>[2x]GPGSTVNEQVQAWESRRPLIQDLARRLLTDDEVLAVTRHCSRYVHEGGVEDLVRPLLAILDRPTKLLLLRDIRSVVAPTDLGRFDSMVMPVELEAFEALKSRAVG

PDZ domain-containing 7 (PDZD7) is part of the ankle-link complex, playing a vital role in the development of cochlear hair cells. The long isoform of PDZD7, which is indispensable for hair cell development, contains tandem PDZ domains (PDZ1-2), an HHD (harmonin homology domain), a PR (proline-rich) region, and a third PDZ domain (PDZ3). The PDZ domains are responsible for interacting with USH2 proteins to form the ankle-link complex. Interestingly, three hearing loss-related proteins (Harmonin, Whirlin, and PDZD7) contain this HHD, but the molecular mechanism of these HHDs is largely unknown.

We then determined the HHD structure at 1.49-Å resolution. The HHD adopts a canonical five-helix fold (α1–α5). In the structure, α1–α5 are aligned anti-parallel to one another, making a five-helix bundle with multiple hydrophobic interactions inside the bundle. The experimental MW of wild-type (WT) PDZD7 (12.1 kDa) matches its theoretical MW of 11.4 kDa, confirming that the PDZD7 HHD is monomeric in solution. Taking these results together, hydrophobic interactions inside the five-helix bundle are important for the folding of the PDZD7 HHD. A unique feature of the PDZD7 HHD structure is that the α1N helix turns back and contacts with the pocket formed between α1, α2, and α4. Val547, Val616, and Trp554 from α1N form extensive hydrophobic interactions with Val577, Cys581, and Val585 from α2, and Ile613 and Val616 from α4. Interestingly, this hydrophobic cleft between α1 and α2 is a common site in HHDs, such as in Harmonin and CCM2, and is required to recognize an isolated amphipathic helix on their binding targets. Structural superimposition of the three structures of PDZD7, harmonin, and CCM2 shows that the PDZD7 HHD is well-aligned onto Harmonin and CCM2, and the α1/α2 cleft of the PDZD7 HHD domain is occupied by α1N and is not available for canonical target recognition. However, the α1/α2 angle in the PDZD7 HHD structure is 25.3°, suggesting that it adopts a more compact conformation.>[2x]MTTTTTKKPHVLVIPFPQSGHMV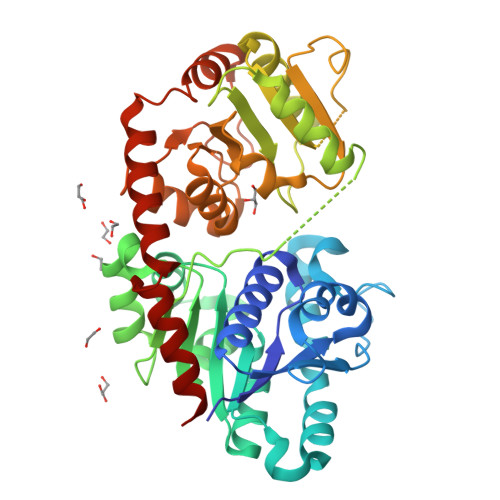PHLDLTHQILLRGATVTVLVTPKNSSYLDALRSLHSPEHFKTLILPFPSHPCIPSGVESLQQLPLEAIVHMFDALSRLHDPLVDFLSRQPPSDLPDAILGSSFLSPWINKVADAFSIKSISFLPINAHSISVMWAQEDRSFFNDLETATTESYGLVINSFYDLEPEFVETVKTRFLNHHRIWTVGPLLPFKAGVDRGGQSSIPPAKVSAWLDSCPEDNSVVYVGFGSQIRLTAEQTAALAAALEKSSVRFIWAVRDAAKKVNSSDNSVEEDVIPAGFEERVKEKGLVIRGWAPQTMILEHRAVGSYLTHLGWGSVLEGMVGGVMLLAWPMQADHFFNTTLIVDKLRAAVRVGENRDSVPDSDKLARILAESAREDLPERVTLMKLREKAMEAIKEGGSSYKNLDELVAEMCL~{N}-[[(2~{R},3~{S},4~{R},5~{R})-5-[8-[3-[[(2~{R},3~{S},4~{R},5~{R})-5-(6-aminopurin-9-yl)-3,4-bis(oxidanyl)oxolan-2-yl]methoxy]prop-1-ynyl]-6-azanyl-purin-9-yl]-3,4-bis(oxidanyl)oxolan-2-yl]methyl]-2-azanyl-ethanesulfonamide 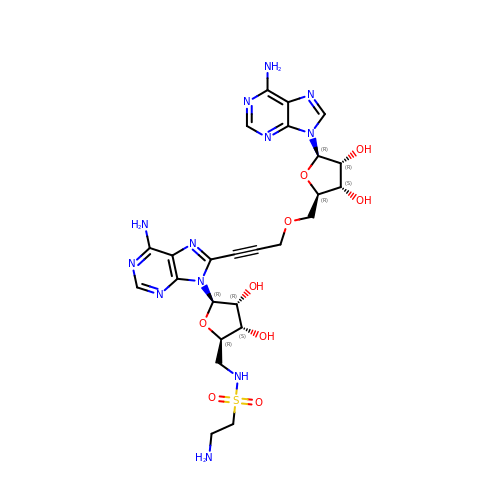| C25 H32 N12 O9 S | BIOOSWGGEOOSLM-AKONZDDMSA-N>[2x]MASPSKAVIVPGNGGGDVTTHGWYGWVKKELEKIPGFQCLAKNMPDPITARESIWLPFMETELHCDEKTIIIGHSSGAIAAMRYAETH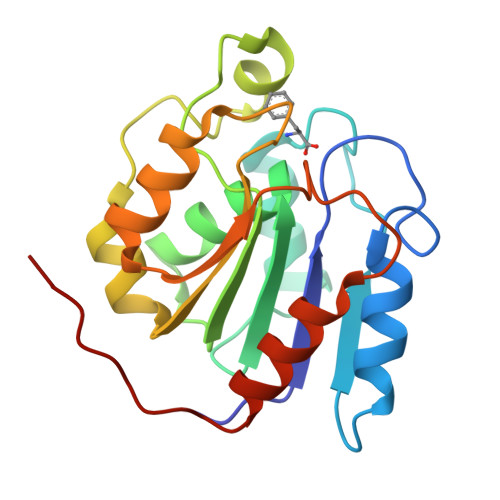RVYAIVLVSAYTSDLGDENERASGYFTRPWQWEKIKANCPYIVQFGSTDDPFLPWKEQQEVADRLETKLHKFTDCGHFQNTEFHELITVVKSLLKVPALEHHHHHH>AAASMSALITENMHMKLYMEGTVNNHHFKCTSEGEGKPYEGTQTMRIKVVEGGPLPFAFDILATSFMYGSKTFINHTQGIPDFFKQSFPEGFTWERVTTYEDGGVLTATQDTSLQDGCLIYNVKIRGVNFPSNGPVMQKKTLGWEACTEMLYPADGGLEGRADMALKLVGGGHLICNLKTTYRSKKPAKNLKMPGVYYVDRRLERIKEADKETYVEQHEVAVARYCDLPSKLAHK[4x]

Fluorescent proteins have facilitated major breakthroughs in modern molecular cell biology. They are widely used for studying biological events, such as cellular trafficking and endocytosis, and have contributed to the development of innovations such as multiphoton microscopy, genetically-encoded sensors, and super-resolution microscopy. mKate, a derivative of eqFP578 from Entacmaea quadricolor, is a bright, monomeric, far-red fluorescent protein with excitation and emission peaks at 588 nm and 635 nm, respectively. Structural characterization of mKate under different conditions revealed the pH-dependent trans-cis isomerization of its chromophore, a discovery that further aided the development of mKate variants with enhanced optical properties. Using a structure-informed approach, we introduced a minimal set of two mutations in the chromophore environment of mKate. The first mutation, S158A, has been shown to destabilize the trans conformation of the chromophore, whereas the second mutation, S143C, was intended to impact the cis conformation.

At high pH (pH 9.0–10.6), this variant appears blue under ambient light, with absorbance and emission maxima shifted to 598 nm and 646 nm, respectively. In the structure of far-red-emitting GmKate (pH 10.0, determined at 1.8 Å resolution), only the cis-conformation of the chromophore was observed. The absorbance peak at 598 nm is indicative of the anionic form of the chromophore, similar to the state observed in mNeptune. Indeed, the π+-π stacking interaction between R197 and the chromophore is conserved at pH 10.0, and may further stabilize the deprotonated state of the chromophore. Chromophore-interacting residues reside in positions similar to those observed at neutral pH. The green (pH 7) to red (pH 10) shift of the absorption energy of GmKate can indeed be attributed to the change in protonation state of the chromophore from neutral at pH 7 to anionic at pH 10. In contrast to mKateS158A and mKate, GmKate has a ∼10 nm red shift in absorbance and emission maxima at pH 10. In the chromophore region, the only difference between mKateS158A and GmKatepH = 10 is the loss of a hydrogen bond due to the substitution of the S143 with a cysteine. This hydrogen bond may stabilize the highest occupied molecular orbital (HOMO) that has electron density concentrated on the phenolate motif. The loss of this hydrogen bond would thus increase the HOMO energy, which results in a decreased energy gap between HOMO and the lowest unoccupied molecular orbital (LUMO), causing a red-shift.>GPGSMKRVVITGMGGVTALGSRWDEIEAALKAGRNAVRRMPDWDYFESLHTRLAAPLPGFAQPADWPRKKTRSMGRVSMYAVRASELALADAGFAGDESISDGRMGVAYGSSSGSVEPIRAFGTMLESGSMTDVTSNSYVQMMPHTTAVNVSLFWDLKGRIVPTSSACASGSQAIGYAYENIAMGKQTLMLAGGAEELSGPAVAVFDTLYATSTRNDEPHLTPRPFDAKRDGLVVGEGAATLVLEEYEHAKARGATIHAEIVGFGCNSDGAHMTQPTASTMARAMQLALEDAKLDANAIAYVNAHGTSTDRGDVAESQATARTFGERMPISSLKSYVGHTLGACGALEAWWTIEMMKRNWYAPTLNLTEVDPACAPLDYIRGEARAIDAEYVMSNNFAFGGINTSLIFRRVR[2x]

Here we report a functional and structural genomics effort that applied saturation-level transposon mutagenesis and next generation sequencing (Tn-seq) to identify essential genes in B. thailandensis, followed by high-throughput structure determination. We used an “ortholog rescue” approach to maximize structural coverage of these gene families, which are likely to be essential not only in B. thailandensis, but also in related, but more virulent, Burkholderia species, such as B. pseudomallei. Using only seven Burkholderia species to select orthologs of essential genes, we solved structures for 49/406 essential gene families, and for 56 total Burkholderia protein targets (including seven ortholog replicates). Of these 56 targets, 25 satisfied criteria for being a potential antimicrobial drug target.

By using an ortholog rescue strategy for insoluble or difficult to crystallize targets, we increased our structural coverage of B. thailandensis essential genes from 31/406 (7.6%) to 49/406 (12.1%). Ortholog structures may also be useful in designing broad-spectrum antibiotics with cross-species activity, and by representing a variety of functionally conservative point mutations in the active site may be useful in developing drugs less susceptible to mutations that cause drug resistance.> AWPKVQPEVNIGVVGHVDHGKTTLVQAITGIWTSKHSEELKRGMTIKLGYAETNIGVCESCKKPEAYVTEPSCKSCGSDDEPKFLRRISFIDAPGHEVLMATMLSGAALMD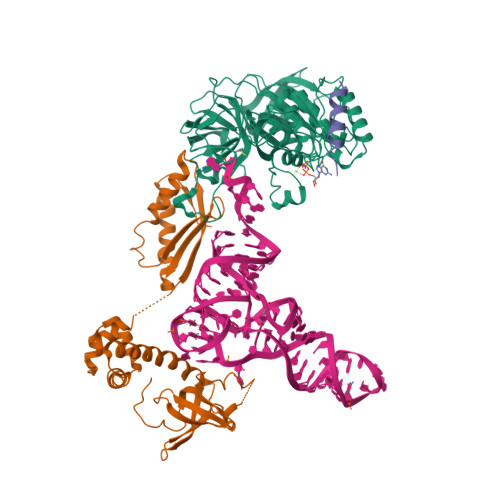GAILVVAANEPFPQPQTREHFVALGIIGVKNLIIVQNKVDVVSKEEALSQYRQIKQFTKGTWAENVPIIPVSALHKINIDSLIEGIEEYIKTPYRDLSQKPVMLVIRSFDVNKPGTQFNELKGGVIGGSIIQGLFKVDQEIKVLPGLRVEKQGKVSYEPIFTKISSIRFGDEEFKEAKPGGLVAIGTYLDPSLTKADNLLGSIITLADAEVPVLWNIRIKYNLLERVVGAKEMLKVDPIRAKETLMLSVGSSTTLGIVTSVKKDEIEVELRRPVAVWSNNIRTVISRQIAGRWRMIGWGLVEI;> MIYSRSKLPSEGEILIATVKQVFDYGSYVSLDEYGGLQAFLPWSEVSSKWVKNIRDVLKENRKVIVKVIRVDRRKGTVDVSLKKVTDDERRKKNLQWKKIQRLDKILELVSQKLKLSEKDAWEQVAWKLEAKYGDPITAIEKAVKEGEKILIDAGVPEIWVKPLLEEASKHAEERKVKMSGLITVRTNEPLGVEKIKEVISKALENIEQDYESLLNIKIYTIGAPRYRVDVVGTNPKEASEALNQIISNLIKIGKEENVDISVVKK;> SSEKEYVEMLDRLYSKLPEKGRKEGTQSLPNMIILNIGNTTIIRNFAEYCDRIRREDKICMKYLLKELAAPGNVDDKGELVIQGKFSSQVINTLMERFLKAYVECSTCKSLDTILKKEKKSWYIVCLACGAQTPVKPL>INQVRPKLPLLKILHAAGAQGEMFTVKEVMHYLGQYIMVKQLYDAAAQHMVYCGGDLLGELLGRQSFSVKDPSPLYD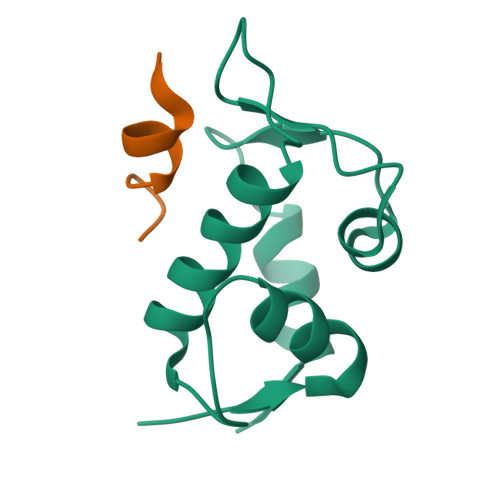MLRKNLVT[4x];>[4x]LTFLEYWAQLMQ> KVTMNDFDYLKLLGKGTFGKVILVREKATGRYYAMKILRKEVIIAKDEVAHTVTESRVLQNTRHPFLTALKYAFQTHDRLCFVMEYANGGELFFHLSRERVFTEERARFYGAEIVSALEYLHSRDVVYRDIKLENLMLDKDGHIKITDFGLCKEGISDGATMKTFCGTPEYLAPEVLEDNDYGRAVDWWGLGVVMYEMMCGRLPFYNQDHERLFELILMEEIRFPRTLSPEAKS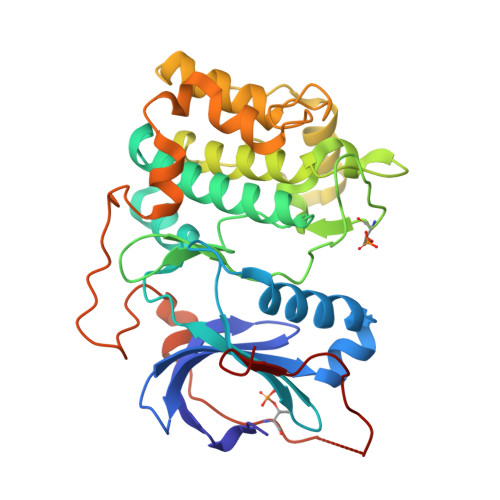LLAGLLKKDPKQRLGGGPSDAKEVMEHRFFLSINWQDVVQKKLLPPFKPQVTSEVDTRYFDDEFTAQSITITPPDRYDSLGLLELDQRTHFPQFDYSASIR4-(3-chlorophenyl)-1H-imidazole | C9 H7 Cl N2 | 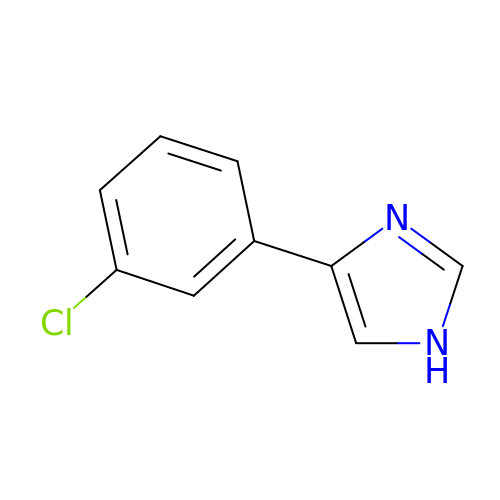YAJYVAFOVNSPBQ-UHFFFAOYSA-N>[12x]MHCPFCRHPDSRVVDSRTTDDGTSIRRRRQCPDCSRRFTTVETCSLMVVKRSGVTEPFSRTKVINGVRKACQGRPVTEDALAQLGQRVEEAVRATGSAELTTHDVGLAILGPLQELDLVAYLRFASVYRAFDSLEDFEAAIAELRETTGHPGEEDDTGAGSQENDRGPTGAGQVPEPAGAADKLAAALEHHHHHH

NrdR, an RNR-specific repressor, controls the transcription of RNR genes and, often, its own, in most bacteria and some archaea. NrdR senses the concentration of nucleotides through its ATP-cone, an evolutionarily mobile domain that also regulates the enzymatic activity of many RNRs, while a Zn-ribbon domain mediates binding to NrdR boxes upstream of and overlapping the transcription start site of RNR genes. NrdRs (140–220 residues) consist of an N-terminal Zn-ribbon domain followed by an ATP-cone domain and in some cases a C-terminal part of variable length and unknown function. In contrast to all earlier suggested mechanisms, we show that the NrdR monomer contains two nucleotide-binding sites, one inner site that binds ATP and one more exposed site that can bind either ATP or dATP.

The structure of ATP-loaded NrdR (2.96 Å resolution from two merged cryo-EM datasets) reveals a dodecameric assembly of three tetramers. In each tetramer, the ATP-cones of chains A and B, and those of chains C and D, interact with each other, respectively. For the Zn-ribbon, the domains of chains A and D and those of chain B and C interact, which generates an intertwined tetrameric structure. In addition, the orientation between the ATP-cone and the Zn-ribbon domains differs by ~90° in chains A and C compared to chains B and D. Perhaps related to these differences, the ATP occupancy in chains B and D is close to 100%, but lower in chains A and C. The described conformational differences allow the tetramers to assemble into a dodecamer, with occluded Zn-ribbon domains, unable to bind DNA. The bases of the outer site nucleotides stack on each other in the ATP-loaded form rather than being sandwiched between the side chains of K69 and V127 and making end-to-end contacts in the dATP/ATP-loaded form. ATP-loaded NrdR forms a dodecamer that cannot bind to DNA.>GMPLDAGGQNSTQMVLAPGASIFRCRQCGQTISRRDWLLPMGGDHEHVV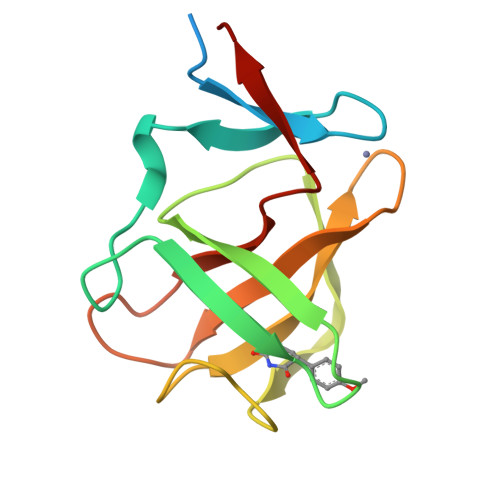FNPAGMIFRVWCFSLAQGLRLIGAPSGEFSWFKGYDWTIALCGQCGSHLGWHYEGGSQPQTFFGLIKDRLAEGPAD[3x]>GSHMIKVLSPAKINLGLWVLGRLPSGYHEILTLYQEIPFYDEIYIREGVLRVETNIGIPQEENLVYKGLREFERITGIEINYSIFIQKNIPPGAGLGGGSSNLAVVLKKVNELLGSPLSEEELRELVGSISADAPFFLLGKSAIGRGKGEVLEPVETEISGKITLVIPQVSSSTGRVYSSLREEHFVTPEYAEEKIQRIISGEVEEIENVLGDIARELYPEINEVYRFVEYLGFKPFVSGSGSTVYFFGGASEELKKAAKMRGWKVVELEL[2x]

4-Diphosphocytidyl-2C-methyl-d-erythritol kinase (IspE) catalyses the ATP-dependent conversion of 4-diphosphocytidyl-2C-methyl-d-erythritol (CDPME) to 4-diphosphocytidyl-2C-methyl-d-erythritol 2-phosphate with the release of ADP. This reaction occurs in the non-mevalonate pathway of isoprenoid precursor biosynthesis and because it is essential in important microbial pathogens and absent from mammals it represents a potential target for anti-infective drugs. The enzyme displays the characteristic α/β galacto-homoserine-mevalonate-phosphomevalonate kinase fold, with the catalytic centre positioned in a deep cleft between the ATP- and CDPME-binding domains. Gel filtration and analytical ultracentrifugation indicate that AaIspE is a monomer in solution.

Similarly, CDPME2P was present in the crystallization conditions for the sample used to derive complex II, but only CDPME was observed. The lack of electron density for the terminal phosphate groups of CDPME2P and AMP-PNP is either a result of disorder and/or hydrolysis. The substrate CDPME binds into a deep cavity between the N- and C-terminal domains, surrounded by residues on β1, α4, the N-terminal end of β2 and θ2 and the β5-β6 loop. His25 forms three hydrogen bonds to the pyrimidine. The cytosine position is also stabilized by hydrophobic contacts with the side chains of Tyr24 and Tyr175, the latter forming π–π stacking interactions with the cytidine. The erythritol moiety of CDPME protrudes into a cavity in which catalytic residues Lys9 and Asp130 are placed. The O2M group, where phosphate addition occurs, participates in hydrogen bonds with Lys9 NZ, Asp130 OD2 and a water molecule (not shown) that in turn associates with the main-chain amide and OG of Ser238, and β-phosphate of ADP. The placement and interactions formed by O2M are consistent with a mechanism that involves polarization of the hydroxyl group and Asp130 acting as a general base in proton abstraction to generate a nucleophile. ADP binds in a cavity formed by the N-terminal domain adjacent to the CDPME-binding site. In AaIspE the syn conformation is also observed with the adenine moiety placed in a hydrophobic cleft surrounded by aliphatic side chains of Ile53, Ile55, Leu61, Ile83 and Lys85 with contributions from Pro89 and Gly96.>GSSVYRIPLADMTFWSWMSYLKELPDIDESRNPILKRLLSGSFLRRDGSTTVNVRVPARELVRLLSLTPEQQREGVSAKVRLINLLDPKYSVYEPYLYREILPKRSPLLLPSLGEYRGAFLTYIFHPLSKGLVGDMLETGRSHPDVQVLAANMVAALKSLHNLGLLHRSIELNSFSVLPDGTVVLGGLDTAAPIGTETRLWVGFFGQETAPEIDRNFLADLALTQGRHTVKSDVYSLGVAFRNLVQLLGNGNLGPEDRGAVRQDHLELLDKLSQKMIEEEPGNRPTIEEIMKDPLFEGLNFEDIEEGKARPFRYKQNRL[6x]

In the present work, we identify a specialized family of kinases that lack the glycine-rich loop that is critical for nucleotide-binding in canonical kinases, leading us to name them the With-No-Gly-loop, or WNG, family. These WNG kinases are conserved throughout the coccidian family of parasites to which Toxoplasma belongs and are secreted into the PV. Like WNG1, BPK1 is secreted into the lumen of the PV and is a clear member of the WNG family. As such, BPK1 shares both primary identity and predicted secondary structure with other WNG kinases throughout its sequence, indicating that its structure would provide faithful insight into the WNG kinase fold.

While we were unable to crystallize an active WNG kinase, we readily obtained crystals of the Toxoplasma pseudokinase BPK1 (bradyzoite pseudokinase 1). We solved the structure of BPK1 to 2.5-Å resolution. The BPK1 structure revealed a divergent kinase fold in which the Gly-loop and the first β-strand that stabilizes it (β1 in PKA nomenclature) have been replaced by a helical extension that packs against the top of the N-lobe of the kinase. Remarkably, not only do the WNG kinases lack a Gly-rich primary sequence, the structural elements that compose the motif have been replaced, resulting in a reorganized N-lobe architecture. The core of the kinase fold, however, is remarkably well conserved, supporting our phylogenetic data, which suggest the WNG family diverged from a canonical Ser/Thr kinase fold. Two salt bridges help stabilize the BPK1 N-lobe within the pseudoactive site, including the bridge between the conserved αC-helix Glu and VAIK-Lys. Notably, the lack of the Gly-loop and β1-strand creates an active site that is much more open than that of a canonical kinase, such as PKA. While BPK1 is a confirmed pseudokinase that cannot bind nucleotide, the other canonical motifs essential for catalysis have been conserved in other WNG family members, suggesting they may be active kinases. To better understand how the WNG kinase active site has adapted to bind nucleotide and catalyze phosphoryl transfer without a Gly-loop, we modeled the WNG1/ROP35 active site using the structure of BPK1 as a template. The rearrangement of the WNG active site has resulted in an unusually open active site that may better accommodate such folded or otherwise sterically restricted substrates.5-methoxy-2-[(5R)-5-methyl-4,5-dihydro-1H-imidazol-2-yl]phenol | C11 H14 N2 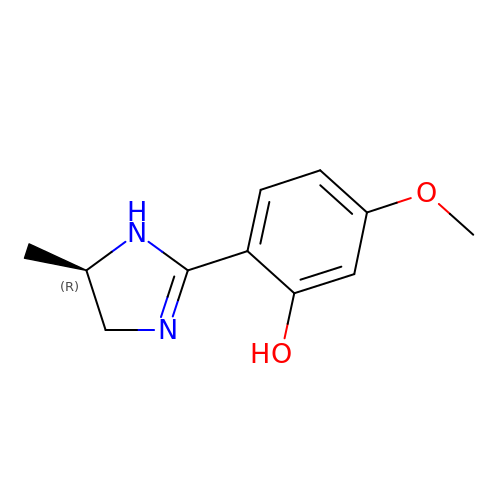O2 | GSHCIAWYWVRHMS-SSDOTTSWSA-N>MAVPFVEDWDLVQTLGEGAY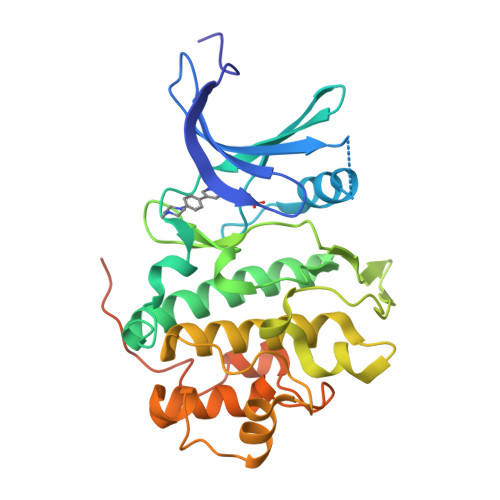GEVQLAVNRVTEEAVAVKIVDMKRAVDCPENIKKEICINKMLNHENVVKFYGHRREGNIQYLFLEYCSGGELFDRIEPDIGMPEPDAQRFFHQLMAGVVYLHGIGITHRDIKPENLLLDERDNLKISDFGLATVFRYNNRERLLNKMCGTLPYVAPELLKRREFHAEPVDVWSCGIVLTAMLAGELPWDQPSDSCQEYSDWKEKKTYLNPWKKIDSAPLALLHKILVENPSARITIPDIKKDRWYNKPLKKGAKRPRVTSGGVSESPSGGHHHHHHHH[2x]> MGPCDIYEAGDTPCVAAHSTTRALYSSFSGALYQLQRGSDDTTTTISPLTAGGIADASAQDTFCANTTCLITIIYDQSGNGNHLTQAPPGGFDGPDTDGYDNLASAIGAPVTLNGQKAYGVFMSPGTGYRNNEATGTATGDEAEGMYAVLDGTHYNDACCFDYGNAETSSTDTGAGHMEAIYLGNSTTWGYGAGDGPWIMVDMENNLFSGADEGYNSGDPSISYRFVTAAVKGG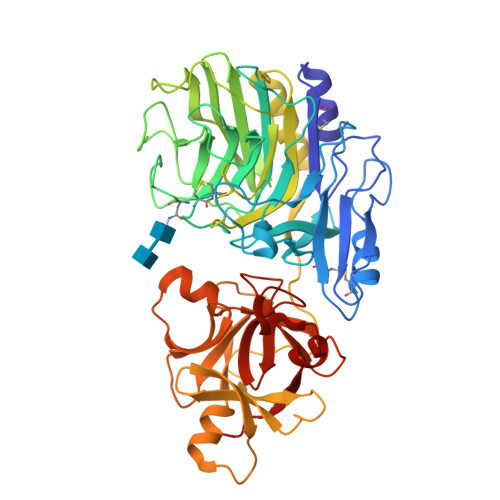ADKWAIRGANAASGSLSTYYSGARPDYSGYNPMSKEGAIILGIGGDNSNGAQGTFYEGVMTSGYPSDDTENSVQENIVAAKYVVGSLVSGPSFTSGEVVSLRVTTPGYTTRYIAHTDTTVNTQVVDDDSSTTLKEEASWTVVTGLANSQCFSFESVDTPGSYIRHYNFELLLNANDGTKQFHEDATFCPQAALNGEGTSLRSWSYPTRYFRHYENVLYAASNGGVQTFDSKTSFNNDVSFEIETAFAS> ADLNWMSEQNAKLAALLNEAELSEKPIEPVRGHIEGGIAQAYAIQQINVQRQLAAGRRVTGRKIGLTSAAVQKQLGVDQPDFGTLFDSMAVNDGEEIAWSRTLQPKCEAEVALVIERDLDHENITLIDLIGATAYALPAIEVVGSRIANWDINILDTVADNASAGLYVLGHTPVKLEGLDLRLAGMVMERAGQQVSLGVGAACLGHPLNAALWL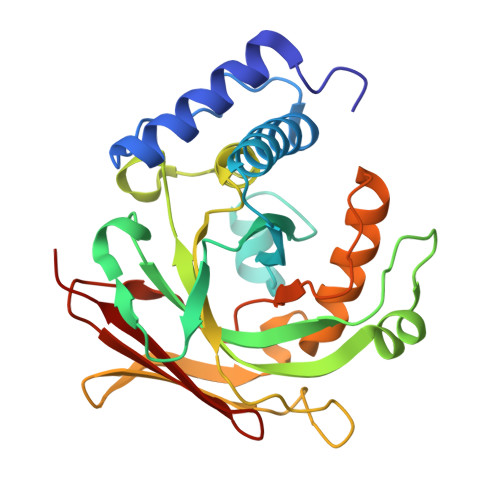ARTLVKQGTPLKSGDVVLSGALGPLVAANPGDVFEARIQGLGSVRACFSPAS> V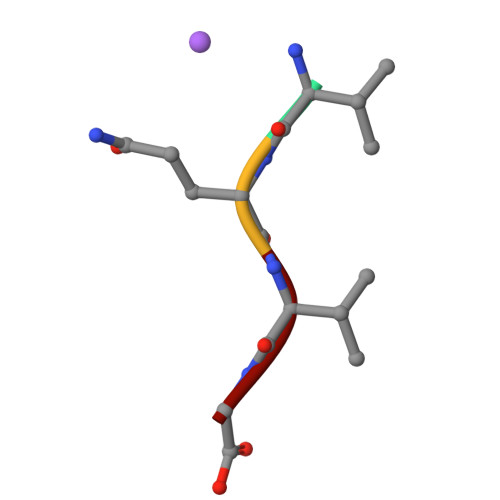QVG> MQNGYTYEDYQDTA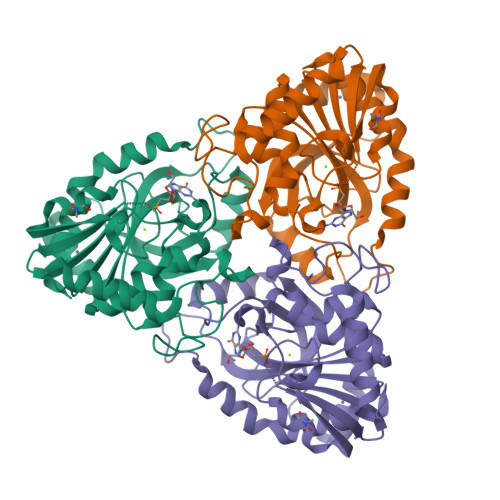KWLLSHTEQRPQVAVICGSGLGGLVNKLTQAQTFDYSEIPNFPESTVPGHAGRLVFGILNGRACVMMQGRFHMYEGYPFWKVTFPVRVFRLLGVETLVVTNAAGGLNPNFEVGDIMLIRDHINLPGFSGENPLRGPNEERFGVRFPAMSDAYDRDMRQKAHSTWKQMGEQRELQEGTYVMLGGPNFETVAECRLLRNLGADAVGMSTVPEVIVARHCGLRVFGFSLITNKVIMDYESQGKANHEEVLEAGKQAAQKLEQFVSLLMASIPVSGHTG>[2x]MVTAFILMVTAAGKEREVMEKLLAMPEVKEAYVVY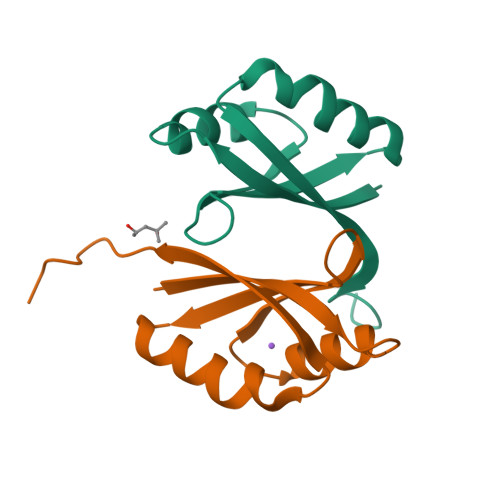GEYDLIVKVETDTLKDLDQFITEKIRKMPEIQMTSTMIAILEHHHHHH Arthrobacter nitroguajacolicus Rü61a 1-H-3-hydroxy-4-oxoquinaldine 2,4-dioxygenase (HOD) and Pseudomonas putida 33/1 1-H-3-hydroxy-4-oxoquinoline 2,4-dioxygenase (QDO) were the first dioxygenases discovered to belong to the ABH-fold family. They catalyze the O2-dependent breakdown of N-heteroaromatic quinolone-type substrates with concomitant carbon monoxide production. Atypical for oxygenases, these enzymes promote the activation of the triplet ground-state O2 molecule without the aid of metal centers or external organic co-factors. Kinetic measurements indicate that their reaction mechanism relies on a fast initial step, during which the substrates' 3-hydroxyl group is deprotonated by the His-Asp subset of the triad, thus promoting its activation for molecular oxygen attack (step 1), whilst the nucleophile is not essential.

However, in contrast with what was observed for the HODH251A–MQO complex, following O2-pressurization (40 bar O2 for 2 minutes) Fourier difference maps revealed a strong elongated peak at the R-site of one of the two HODS101A chains in the asymmetric unit. Modelling of this peak as an O2 molecule did not result in negative difference density, and occupancy refinement converged to unity with atomic displacement parameters for both oxygen atoms consistent with those of the surrounding atoms (average B-value MQO = 21.3 Å2, B-value O2(O1) = 20.5 Å2 and B-value O2(O2) = 19.7 Å2). Moreover, omit maps for the individual oxygen atoms produced difference Fourier peaks, supporting the assignment as O2. The equivalent peak in the other protein chain was less prominent and more spherical in shape. We have modelled this peak also as O2 and occupancy refinement converged at 0.80 with an average B-value of 30.3 Å2. Using the fully occupied O2 molecule as a reference, we find that dioxygen binds underneath the A-ring of MQO approximately parallel to its plane at an average distance of 3.2 Å. The ligand's atoms closest to O2(O2) and O2(O1) are C2 at 3.1 Å and C4 at 3.4 Å, respectively, and dioxygen further interacts with the main chain amide groups of W36 and H102 as well as with the side chain of the latter residue. The O2 molecular axis is roughly parallel to the MQO(C2–C4) direction as quantified by the dihedral angle Φ(C4–C2–O2–O1) of −2.2°. Thus, in the HODS101A–MQO–O2 ternary complex, dioxygen appears to preferentially adopt an orientation that mimics that of the endoperoxide during the catalytic cycle (step 4 in Fig. 1B).

>[2x]MRGSHHHHHHGSMTDTYLHETLVFDNKLSYIDNQRDTDGPAILLLPGWCHDHRVYKYLIQELDADFRVIVPNWRGHGLSPSEVPDFGYQEQVKDALEILDQLGVETFLPVSHAHGGWVLVELLEQAGPERAPRGIIMDWLMWAPKPDFAKSLTLLKDPERWREGTHGLFDVWLDGHDEKRVRHHLLEEMADYGYDCWGRSGRVIEDAYGRNGSPMQMMANLTKTRPIRHIFSQPTEPEYEKINSDFAEQHPWFSYAKLGGPTHFPAIDVPDRAAVHIREFATAIRQGQ PfHK is the first and simultaneously rate-limiting enzyme of glycolysis, catalyzing the phosphorylation of glucose to glucose-6-phosphate (G6P). ATP provides the phosphoryl group and the reaction requires divalent cations, usually Mg2+. The overall fold of each monomer is similar to that of other hexokinases and consists of two domains: a small domain comprising residues E94-L239 and a large domain comprising residues M1-Q93 and N240-P490, with the active site located between both domains. As already discussed by Srivastava and colleagues, the tetrameric assembly of Plasmodium hexokinases is unique since most hexokinases occur in a biologically relevant manner as monomers or (pseudo-)dimers.

In this study, we present the first PfHK structure in a closed-state conformation complexed with glucose. The crystals belonged to space group P3121 and contained two monomers within the asymmetric unit. The active site of both monomers contained a glucose molecule and, in one monomer, a citrate molecule was additionally bound. The citrate interacts with conserved residues from both domains: G104, N107, R109, T268, and S436, which are typically involved in ADP/ATP binding. In monomer B, P-insert residues L130-G141 adopt a completely different conformation compared to monomer A, pointing into the active site channel and resulting in a large shift of up to 20 Å for residues G134-E139. In subunit B, the P-insert occupied the ATP-binding site via interactions with the large domain, thus inhibiting ATP binding and causing the C-loop and P-insert to adopt a pre- or post-catalytic conformation. The citrate molecule was bound to the phosphate binding and transfer site of subunit A. Thus, it forced a rearrangement of the C-loop in this subunit, followed by a rearrangement of the P-insert, resulting in a catalytically active conformation of both loops. The P-insert is rearranged in our structure upon citrate binding and probably also upon ATP binding. This movement is responsible for the loss of multiple contacts between the small and large domains in monomer A. Of particular importance appears to be the interaction between the P-insert residues L130-S135 (small domain) and region P304-Y312 (large domain), which, in turn, is part of the AB interface. The loss of this contact alters the AB interface and affects the neighboring molecule in the tetramer. This could be an allosteric effect, possibly explaining the binding of citrate (or physiologically ATP) only to one subunit.

>[2x]MSEYDIAKNDVTYTKLDTIECDIPINEELSWRINKFVNQLRISYSTLEEFVDNFVYELKKGLEAHRKHPNLWIPHECSFKMLDSCIANIPTGQEKGTYYAIDFGGTNFRAVRASLDGKGKIKRDQETYSLKFTGSYSHEKGLLDKHATASQLFDHFAERIKYIMGEFNDLDNKEVKSVGFTFSFPCTSPSINCSILIDWTKGFETGRATNDPVEGRDVCKLMNDAFVRAAIPAKVCCVLNDAVGTLMSCAYQKGRGTPPCYIGIILGTGSNGCYYEPEWKKYKYAGKIINIEFGNFDKDLPTSPIDLVMDWYSANRSRQLFEKMISGAYLGEIVRRFMVNVLQSACSKKMWISDSFNSESGSVVLNDTSKNFEDSRKVAKAAWDMDFTDEQIYVLRKICEAVYNRSAALAAGTIAAIAKRIKIIEHSKFTCGVDGSLFVKNAWYCKRLQEHLKVILADKAENLIIIPADDGSGKGAAITAAVIALNADIPQLP6-(4-benzoylphenyl)-1-(pyridin-4-ylmethyl)-1H-pyrazolo[3,4-b]pyridine-4-carboxylic 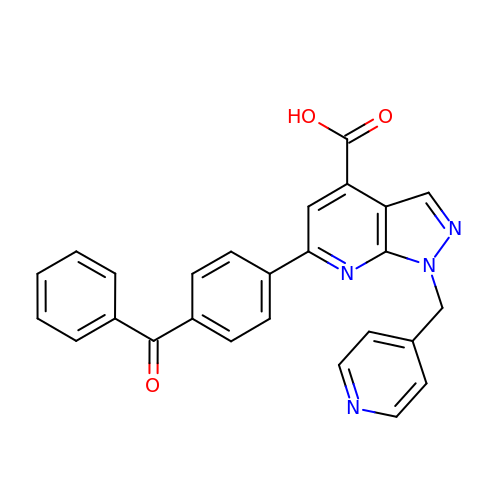acid | C26 H18 N4 O3 | PTCVSDDJAQNAKH-UHFFFAOYSA-N> EHRGPPPEYPFK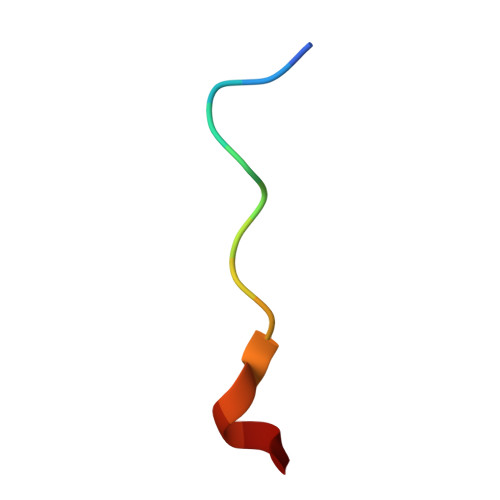GM>MRGSHHHHHHGSELPQMTQQLNSDDMQEQLSATRKFSQILSDGNEQIQAVIDAGALPALVQLLSSPNEQILQEALWALSNIASGGNEQIQAVIDAGALPALVQLLSSPNEQILQEALWALSNIASGGNEQIQAVIDAGALPALVQLLSSPNEQILQEALWALSNIASGGNEQKQAVKEAGALEKLEQLQSHENEKIQKE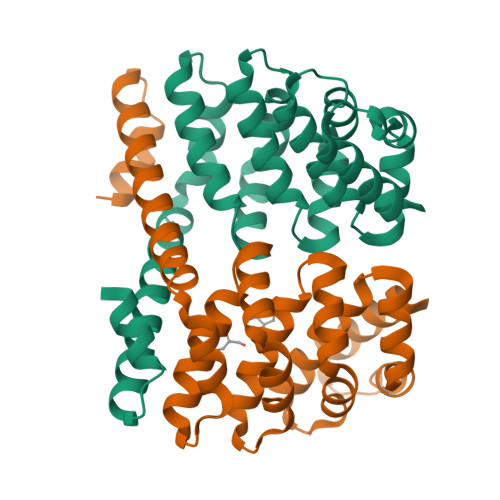AQEALEKLQSH[4x]>WEECFQAAVQLALRAGQIIRKALTEEKRVSTKTSAADLVTETDHLVEDLIISELRERFPSHRFIAEEAAASGAKCVLTHSPTWIIDPIDGTCNFVHRFPTVAVSIGFAVRQELEFGVIYHCTEERLYTGRRGRGAFCNGQRLRVSGETDLSKALVLTEIGPKRDPATLKLFLSNMERLLHAKAHGVRVIGSSTLALCHLASGAADAYYQFGLHCWDLAAATVIIREAGGIVIDTSG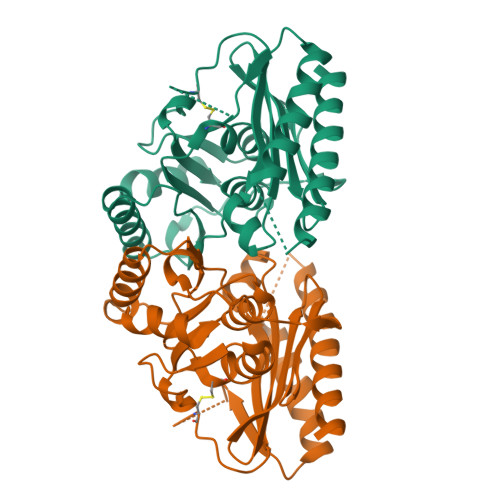GPLDLMACRVVAASTREMAMLIAQALQTINYGRDDEK[4x]cyanic acid 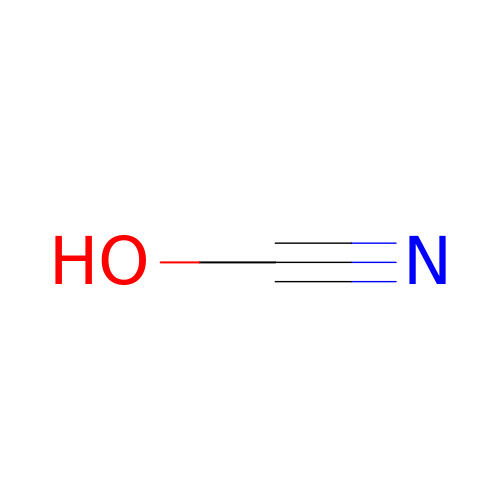| C H N O | XLJMAIOERFSOGZ-UHFFFAOYSA-N> AMPFEIEVLLPGEISPAETSALQKCEGKIITFSTLRHRASLVDIALSSYYINGAPPDT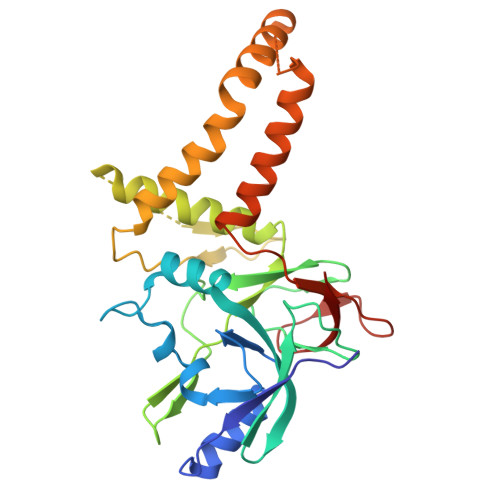LSLLEAYRMRFAAVITRVIPGKLLAHAIGVGTPTPGLFIQNTSPVDLCNGDYICLLPPVFGSADEIRLDSVGLEIVFPLTIPQTLMREIIAKVVARAVERTAADVICYNGRRYELETNLQHRDGSDAAIRTLVLNLMFSINEGTTLILTLITRLLRFPIYEAISSWISTSSRLGDTLGTRAILRVCVFDGPSTVHPGDRTAVIQV1-[5-(trifluoromethyl)furan-2-yl]methanamine | C6 H6 F3 N O | 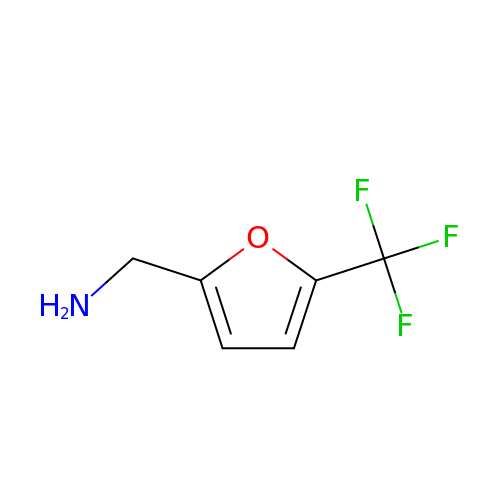MMOMFJIMQXUJMQ-UHFFFAOYSA-N The prototypical m6A-dependent endonuclease R.DpnI was originally isolated from Streptococcus pneumoniae. The biological activity is due to the specificity of R.DpnI for Dam-methylated (Gm6ATC) sites. R.DpnI cleaves its target sequence with high efficiency if both DNA strands are methylated and with lesser efficiency if only one strand is modified. We have shown that the enzyme is a type IIE restriction endonuclease and consists of an N-terminal catalytic domain of the PD-(D/E)XK type (residues 1-182) and a C-terminal winged helix domain (residues 183-254).

We present a crystal form of R.DpnI with one molecule of the enzyme and two target DNA duplexes in the asymmetric unit. One oligoduplex is bound to the winged helix domain as previously reported. The other duplex binds to the catalytic domain in a conformation that is posed for cleavage. However, the relative domain orientations differ drastically between the two structures [according to the DynDom server the change can be described as a 75°–80° rotation]. The catalytic region of R.DpnI is disordered in the absence of the substrate, but folds upon DNA binding and forms a standard PD-(D/E)XK active site with two binding sites for divalent cations. Based on the anomalous X-ray diffraction signal, we suspect that one of the sites (site 1) is nearly fully occupied by a Ca2+ ion, while the other site (site 2) may be occupied by a mixture of Ca2+ and Na+ ions. The site 1 Ca2+ ion is hexacoordinated by the side chains of Asp53 (the ‘bridging’ ligand) and Glu64, as well as by the main chain carbonyl oxygen atom of Leu65, the proS (OP2) non-bridging oxygen of the ‘scissile’ phosphate, and two water molecules. A three-stranded antiparallel β-sheet with a long loop (residues 75-80 and 123-144) wedges into the major groove of the target DNA. The hydrophobic pocket is formed by Leu129, Arg135 and Trp138, which are all located in the long loop that gets ordered upon DNA binding. It simultaneously interacts with both methyl groups: its pyrrole ring is in van der Waals contact with the m6A of the proximal DNA strand and its benzene ring with the m6A of the distal strand.

> GPHMELHFNLELVETYKSNSQKARILTEDWVYRQSYCPNCGNNPLNHFENNRPVADFYCNHCSEEFELKSKKGNFSSTINDGAYATMMKRVQADNNPNFFFLTYTKNFEVNNFLVLPKQFVTPKSIIQRKPLAPTANRAGWIGCNIDLSQVPSKGRIFLVQDGQVRDPEKVTKEFKQGLFLRKSSLSSRGWTIEILNCIDKIEGSEFTLEDMYRFESDLKNIFVKNNHIKEKIRQQLQILRDKEIIEFKGRGKYRKL>MAPFEIPDRYKKPA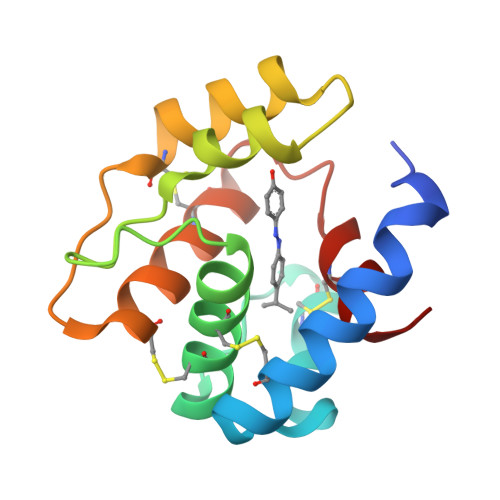KMLHEICIAESGASEEQLRTCLDGTVPTAPAAKCYIHCLFDKIDVVDEATGRILLDRLLYIIPDDVKAAVDHLTRECSHIVTPDKCETAYETVKCYFNAHDEVIKFCHLLVLE[2x]> PISPIETVPVKLKPGMDGPKVKQWPLTEEKIKALVEICTEMEKEGKISKIGPENPYNTPVFAIKKKDSTKWRKLVDFRELNKRTQDFWEVQLGIPHPAGLKKKKSVTVLDVGDAYFSVPLDEDFRKYTAFTIPSINNETPGIRYQYNVLPQGWKGSPAIFQSSMTKILEPFRKQNPDIVIYQYMDDLYVGSDLEIGQHRTKIEELRQHLLRWGLTTP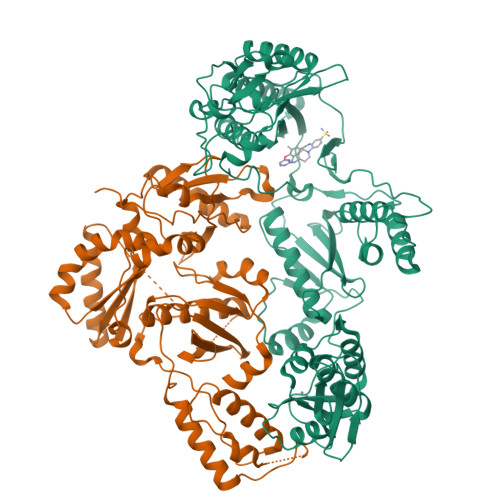DKKHQKEPPFLWMGYELHPDKWTVQPIVLPEKDSWTVNDIQKLVGKLNWASQIYPGIKVRQLCKLLRGTKALTEVIPLTEEAELELAENREILKEPVHGVYYDPSKDLIAEIQKQGQGQWTYQIYQEPFKNLKTGKYARMRGAHTNDVKQLTEAVQKITTESIVIWGKTPKFKLPIQKETWETWWTEYWQATWIPEWEFVNTPPLVKLWYQLEKEPIVGAETFYVDGAANRETKLGKAGYVTNRGRQKVVTLTDTTNQKTELQAIYLALQDSGLEVNIVTDSQYALGIIQAQPDQSESELVNQIIEQLIKKEKVYLAWVPAHKGIGGNEQVDKLVSAGIRKVLF;> PISPIETVPVKLKPGMDGPKVKQWPLTEEKIKALVEICTEMEKEGKISKIGPENPYNTPVFAIKKKDSTKWRKLVDFRELNKRTQDFWEVQLGIPHPAGLKKKKSVTVLDVGDAYFSVPLDEDFRKYTAFTIPSINNETPGIRYQYNVLPQGWKGSPAIFQSSMTKILEPFRKQNPDIVIYQYMDDLYVGSDLEIGQHRTKIEELRQHLLRWGLTTPDKKHQKEPPFLWMGYELHPDKWTVQPIVLPEKDSWTVNDIQKLVGKLNWASQIYPGIKVRQLCKLLRGTKALTEVIPLTEEAELELAENREILKEPVHGVYYDPSKDLIAEIQKQGQGQWTYQIYQEPFKNLKTGKYARMRGAHTNDVKQLTEAVQKITTESIVIWGKTPKFKLPIQKETWETWWTEYWQATWIPEWEFVNTPPLVKLWYQLEKEPIVGAETF>SNAARDNVTKSKISQYKDQIFDLTYPYSGNENSSVIAVGFLDYSCGHCKAIKNDIKQLINDGKIKYIFRDAPILGNASLKAAKSALAVYFLDKEKYFDFHHAALSHKGEFSDESILDIVKNIGIDEDDFND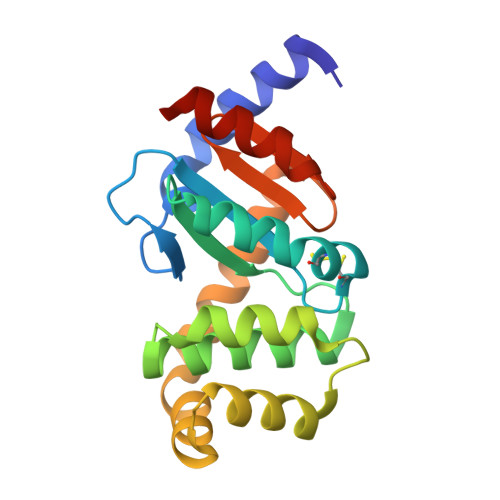SIKDNADKIEQMINNSRLLVRDLGVGGTPFLIIGDSLFVGATDLNVLRKKVDELSHKQG[4x]> MTHPDPTLFGHDPWWLMLAKAVAIFVFLLLTVLSAILIERKLLGRMQMRFGPNRVGPAGLLQSLADGIKLALKEGLVPAGVDKPIYLLAPVISVIPAFVAFSV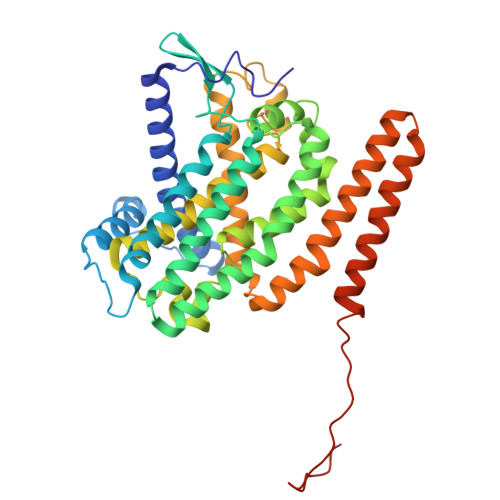IPLGGAVSVFGHRTPLQLTDLPVAVLFILAATSIGVYGIVLAGWASGSTYPLLGGLRSSAQVVSYEIAMGLSFVAVFLYAGTMSTSGIVAAQDRTWFVFLLLPSFLVYVVSMVGETNRAPFDLPEAEGELVGGFHTEYSSLKFAMFMLAEYVNMTTVSALATTMFLGGWHAPFPFNLIDGANSGWWPLLWFTAKVWTFMFLYFWLRATLPRLRYDQFMALGWKVLIPVSLLWIMVVAITRSLRQHGEGTWAAWLLTAAVVVVVALIWGLATSLRRRTVQPPPPQSTGAYPVPPLPSVGTKETADA> CYHKFAHKPPISSAEMTFRRPAQAFPVSYSSSGARRPSLDSMENQVSVDAFKILEDPKWEFPRKNLVLGKTLGEGEFGKVVKATAFHLKGRAGYTTVAVKMLKENASPSELRDLLSEFNVLKQVNHPHVIKLYGACSQDGPLLLIVEYAKYGSLRGFLRESRKVGPGYLGSGGSRNSSSLDHPDERALTMGDLISFAWQISQGMQYLAEMKLVHRDLAARNILVAEGRKMKISDFGLSRDVY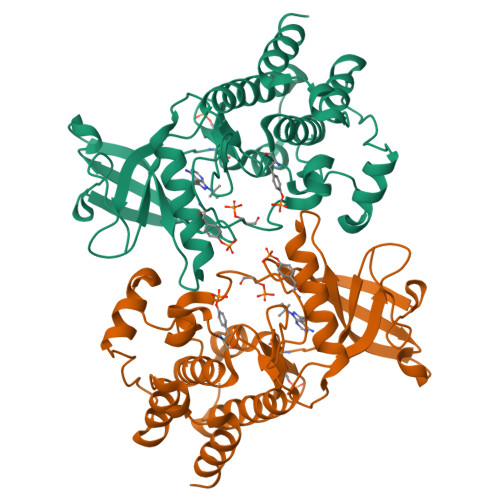EEDSYVKRSQGRIPVKWMAIESLFDHIYTTQSDVWSFGVLLWEIVTLGGNPYPGIPPERLFNLLKTGHRMERPDNCSEEMYRLMLQCWKQEPDKRPVFADISKDLEKMMVKRR> GSHMAVLQKSSPLQENKDFYILDTHTQKKISFEDMILELLKADVILLGEKHDEVKHKISQVMIFNALEGNLSSQNINFDVALEMLASTEQNHLDKAFKNKKTIKANELTNALNWDKVWKWKDYEQFVNVVFYSKSKILGANLSRSEITSIYNGAQPLKGYVSTTNEVKKQLFDIISLSHKLNPEENKELLDKLVEIQQFKDRRMADVLVHHVNKVLLLAGSYHTSKK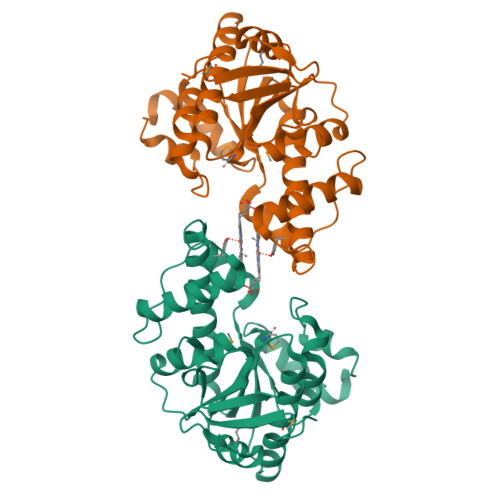IGIPLHIQDFKSSKKIVVVNLSYGEIDLKDSDYVLIYKGEE>YPEESEKRKRVSSAVQFLHDSRVKITPAANKIQFLKSKGLTTEEVCE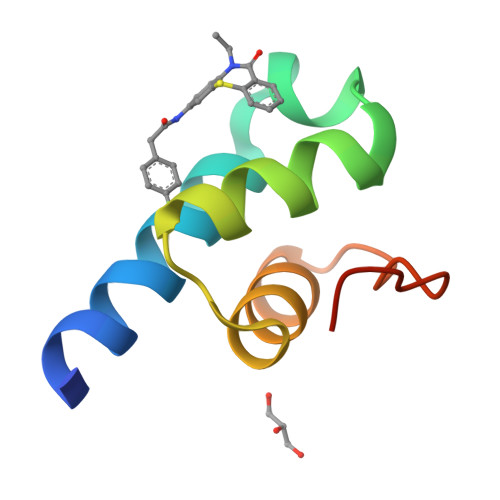AFEKAGQTIPLDEIKKIMN[2x]>MSLILCIDVGNSHIYGGVFDGDEIKLRFRHTSKVSTSDELGIFLKSVLRENNCSPETIRKIAICSVVPQVDYSLRSACVKYFSIDPFLLQAGVKTGLNIKYRNPVEVGADRIANAIAATHSFPNQNIIVIDFGTATTFCAISHKKAYLGGAILPGLRLSADALSKNTAKLPSVEIIKTESVVGRSTIESIQSGVYYGVLGACKELIQRIHHEAFNGDQILILATGGFASLFDKQGLYDHLVPDLVLQGIRLAAMMNTAEGHHHH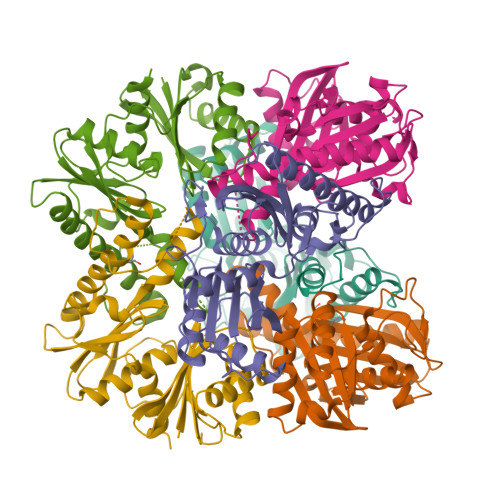HH[12x]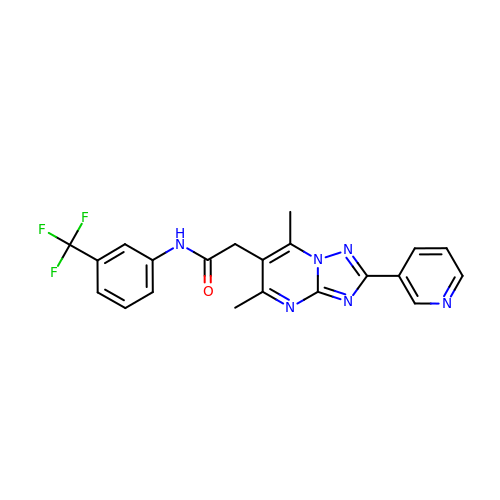2-[5,7-dimethyl-2-(pyridin-3-yl)[1,2,4]triazolo[1,5-a]pyrimidin-6-yl]-N-[3-(trifluoromethyl)phenyl]acetamide | C21 H17 F3 N6 O | MTJCWZPTCSKXKK-UHFFFAOYSA-N> MHYLPVAIVTGATRGIGKAICQKLFQKGLSCIILGSTKESIERTAIDRGQLQSGLSYQRQCAIAIDFKKWPHWLDYESYDGIEYFKDRPPLKQKYSTLFDPCNKWSNNERRYYVNLLIN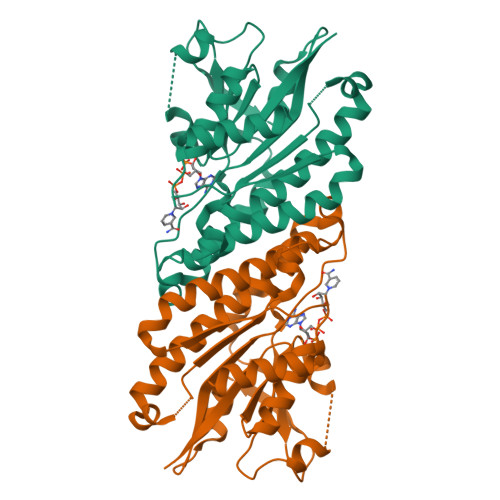CAGLTQESLSVRTTASQIQDIMNVNFMSPVTMTNICIKYMMKSQRRWPELSGQSARPTIVNISSILHSGKMKVPGTSVYSASKAALSRFTEVLAAEMEPRNIRCFTISPGLVKGTDMIQNLPVEAKEMLERTIGASGTSAPAEIAEEVWSLYSR> QSHLPMPTTPYDTILKAGVVLQLFSHPGAGKTRAIPEYVRQLMTWSNRVYVAGPTRVVAREMLESLQGTKWVCAMVKGLPRPHALARVVVTTHQTLLRYALTSGLLFAKDVSYVLDETHVDSAHTKVLRALIH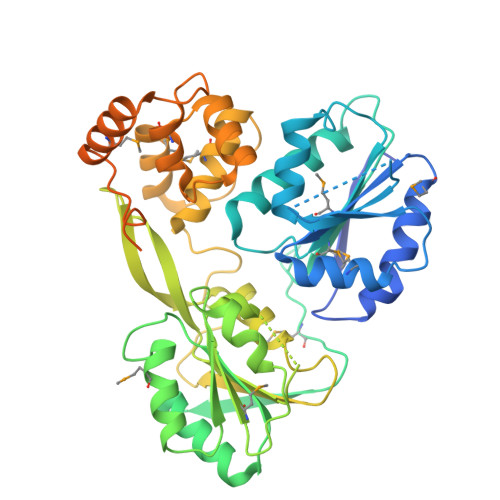QTVCKEKSKAACIEMTATGRDSTTGEVRVSMDSNYPIVDRVYNEGVVQAVRKYAETHGPARVAVFVPGLTGKNGALMVAKHIKQTTPYTTIVLSRKTYERNIKLVFKQYPRGMCVVTTSISECGANYDLDAVFDTCQQYHYLVTAVGTKGVITPSTQAQTCQRRGRIGRRREGGYYRPANYDITQAPVLDHPDSVTLLEANMCLRALDLPEEPCGAAVQQAMLRLQPSKDQVYRWLTEQDTETLTEAMAIYSAEGGRRSREQERAIRNRMRSYFNDARWERVEDDAELPAVSPGEYIRDEEGTEVIAGASYVQAPPPYRVRVNQATLLRGSDVKALREEGDRDLAAAIRDEIPEPT> ANSVCFTFTDFESGQQDLIFQGDASVGSNKALQLTKVDSKGNPQGGSVGRALYTAPIRLWQSSSLVASFETTFTFSISQGSSTPADALTFFIASPDTKIPSGSGGRLLGLFGSSNNAGSDNGVVSVEFDTYPNTDIGDPNYRHIGIDV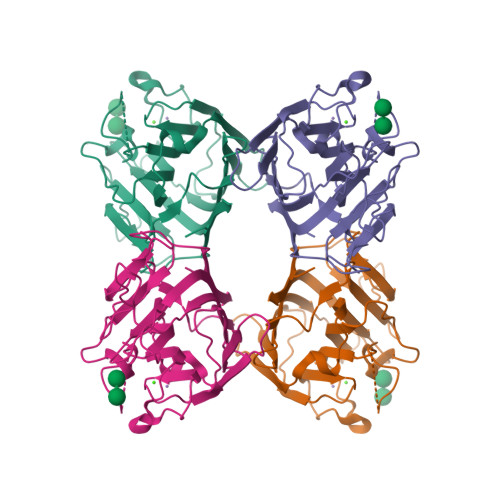NSIRSKAASKWDWQNGKTATAHISYNSASKRLSVVSSYPNSSPVVVSFDVELNNVBPBWVRVGFSATTGQYTQTNNILAWSFRSSLMGYQAN> MQSSPSPAHPQLPVLQTQMVSDGMTGSNPVSPASSSSPASSGAGGISPQHIAQDSSLDGPPGPPDGATVPLEGFSLSQAADLANKGPKWEKSHAEIAEQAKHEAEIETRIAELRKEGFWSLKRLPKVPEPPRPKGHWDYLCEEMQWLSADFAQERRWKRGVARKVVRMVIRHHEEQRQKEERARREEQAKLRRIASTMAKDVRQFWSNVEKVVQFKQQSRLEEKRKKALDLHLDFIVGQTEKYSDLLSQSLNQPLTSSKAGSSPCLGSSSAASSPPPPASRLDDEDGDFQPQEDEEEDDEETIEVEEQQEGNDAEAQRREIELLRREGELPLEELLRSLPPQLLEGPSSPSQTPSSHDSDTRDGPEEGAEEEPPQVLEIKPPPSAVTQRNKQPWHPDEDDEEFTANEEEAEDEEDTIAAEEQLEGEVDHAMELSELAREGELSMEELLQQYAGAYAPGSGSSEDEDEDEVDANSSDCEPEGPVEAEEPPQEDSSSQSDSVEDRSEDEEDEHSEEEETSGSSASEESESEESEDAQSQSQADEEEEDDDFGVEYLLARDEEQSEADAGSGPPTPGPTTLGPKKEITDIAAAAESLQPKGYTLATTQVKTPIPLLLRGQLREYQHIGLDWLVTMYEKKLNGILADEMGLGKTIQTISLLAHLACEKGNWGPHLIIVPTSVMLNWEMELKRWCPSFKILTYYGAQKERKLKRQGWTKPNAFHVCITSYKLVLQDHQAFRRKNWRYLILDEAQNIKNFKSQRWQSLLNFNSQRRLLLTGTPLQNSLMELWSLMHFLMPHVFQSHREFKEWFSNPLT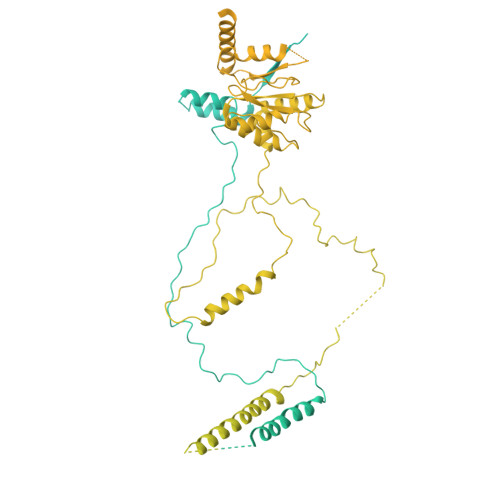GMIEGSQEYNEGLVKRLHKVLRPFLLRRVKVDVEKQMPKKYEHVIRCRLSKRQRCLYDDFMAQTTTKETLATGHFMSVINILMQLRKVCNHPNLFDPRPVTSPFITPGICFSTASLVLRATDVHPLQRIDMGRFDLIGLEGRVSRYEADTFLPRHRLSRRVLLEVATAPDPPPRPKPVKMKVNRMLQPVPKQEGRTVVVVNNPRAPLGPVPVRPPPGPELSAQPTPGPVPQVLPASLMVSASPAGPPLIPASRPPGPVLLPPLQPNSGSLPQVLPSPLGVLSGTSRPPTPTLSLKPTPPAPVRLSPAPPPGSSSLLKPLTVPPGYTFPPAAATTTSTTTATATTTAVPAPTPAPQRLILSPDMQARLPSGEVVSIGQLASLAQRPVANAGGSKPLTFQIQGNKLTLTGAQVRQLAVGQPRPLQRNVVHLVSAGGQHHLISQPAHVALIQAVAPTPGPTPVSVLPSSTPSTTPAPTGLSLPLAANQVPPTMVNNTGVVKIVVRQAPRDGLTPVPPLAPAPRPPSSGLPAVLNPRPTLTPGRLPTPTLGTARAPMPTPTLVRPLLKLVHSPSPEVSASAPGAAPLTISSPLHVPSSLPGPASSPMPIPNSSPLASPVSSTVSVPLSSSLPISVPTTLPAPASAPLTIPISAPLTVSASGPALLTSVTPPLAPVVPAAPGPPSLAPSGASPSASALTLGLATAPSLSSSQTPGHPLLLAPTSSHVPGLNSTVAPACSPVLVPASALASPFPSAPNPAPAQASLLAPASSASQALATPLAPMAAPQTAILAPSPAPPLAPLPVLAPSPGAAPVLASSQTPVPVMAPSSTPGTSLASASPVPAPTPVLAPSSTQTMLPAPVPSPLPSPASTQTLALAPALAPTLGGSSPSQTLSLGTGNPQGPFPTQTLSLTPASSLVPTPAQTLSLAPGPPLGPTQTLSLAPAPPLAPASPVGPAPAHTLTLAPASSSASLLAPASVQTLTLSPAPVPTLGPAAAQTLALAPASTQSPASQASSLVVSASGAAPLPVTMVSRLPVSKDEPDTLTLRSGPPSPPSTATSFGGPRPRRQPPPPPRSPFYLDSLEEKRKRQRSERLERIFQLSEAHGALAPVYGTEVLDFCTLPQPVASPIGPRSPGPSHPTFWTYTEAAHRAVLFPQQRLDQLSEIIERFIFVMPPVEAPPPSLHACHPPPWLAPRQAAFQEQLASELWPRARPLHRIVCNMRTQFPDLRLIQYDCGKLQTLAVLLRQLKAEGHRVLIFTQMTRMLDVLEQFLTYHGHLYLRLDGSTRVEQRQALMERFNADKRIFCFILSTRSGGVGVNLTGADTVVFYDSDWNPTMDAQAQDRCHRIGQTRDVHIYRLISERTVEENILKKANQKRMLGDMAIEGGNFTTAYFKQQTIRELFDMPLEEPSSSSVPSAPEEEEETVASKQTHILEQALCRAEDEEDIRAATQAKAEQVAELAEFNENDGFPAGEGEEAGRPGAEDEEMSRAEQEIAALVEQLTPIERYAMKFLEASLEEVSREELKQAEEQVEAARKDLDQAKEEVFRLPQEEEEGPGAGDESSCGTGGGTHRRSKKAKAPERPGTRVSERLRGARAETQGANHTPVISAHQTRSTTTPPRCSPARERVPRPAPRPRPTPASAPAAIPALVPVPVSAPVPISAPNPITILPVHILPSPPPPSQIPPCSSPACTPPPACTPPPAHTPPPAQTCLVTPSSPLLLGPPSVPISASVTNLPLGLRPEAELCAQALASPESLELASVASSETSSLSLVPPKDLLPVAVEILPVSEKNLSLTPSAPSLTLEAGSIPNGQEQEAPDSAEGTTLTVLPEGEELPLCVSESNGLELPPSAASDEPLQEPLEADRTSEELTEAKTPTSSPEKPQELVTAEVAAPSTSSSATSSPEGPSPARPPRRRTSADVEIRGQGTGRPGQPPGPKVLRKLPGRLVTVVEEKELVRRRRQQRGAASTLVPGVSETSASPGSPSVRSMSGPESSPPIGGPCEAAPSSSLPTPPQQPFIARRHIELGVTGGGSPENGDGALLAITPPAVKRRRGRPPKKNRSPADAGRGVDEAPSSTLKGKTNGADPVPGPETLIVADPVLEPQLIPGPQPLGPQPVHRPNPLLSPVEKRRRGRPPKARDLPIPGTISSAGDGNSESRTQPPPHPSPLTPLPPLLVCPTATVANTVTTVTISTSPPKRKRGRPPKNPPSPRPSQLPVLDRDSTSVLESCGLGRRRQPQGQGESEGSSSDEDGSRPLTRLARLRLEAEGMRGRKSGGSMVVAVIQDDLDLADSGPGGLELTPPVVSLTPKLRSTRLRPGSLVPPLETEKLPRKRAGAPVGGSPGLAKRGRLQPPSPLGPEGSVEESEAEASGEEEEGDGTPRRRPGPRRLVGTTNQGDQRILRSSAPPSLAGPAVSHRGRKAKT>SGFVCNTCPEKWINFQRKCYYFGKGTKQWVHARYACDDMEGQLVSIHSPEEQDFLTKHASHTGSWIGLRNLDLKGEFIWVDGSHVDYSNWAPGEP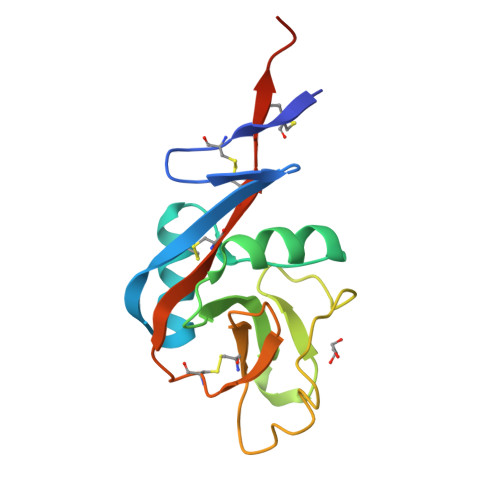TSRSQGEACVMMRGSGRWNDAFCDRKLGAWVCDRLATCTPPASEGSAE[8x]Diperodon (S-enantiomer) 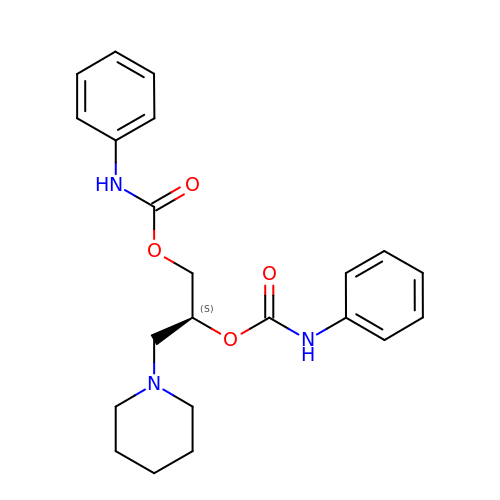| C22 H27 N3 O4 | YUGZHQHSNYIFLG-FQEVSTJZSA-N> PQLPEVETIRRTLLPLIVGKTIEDVRIFWPNIIRHPRDSEAFAARMIGQTVRGLERRGKFLKFLLDRDALISHLRMEGRYAVASALEPLEPHTHVVFCFTDGSELRYRDVRKFGTMHVYAKEEADRRPPLAELGPEPLSPAFSPAVLAERAVKTK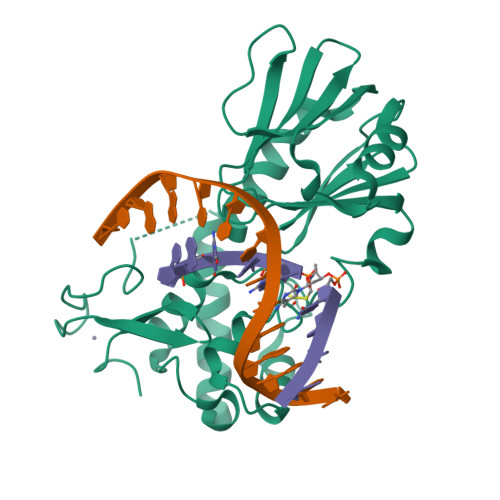RSVKALLLDCTVVAGFGNIYVDESLFRAGILPGRPAASLSSKEIERLHEEMVATIGEAVMKGGSTPRTYVNTQGEAGTFQHHLYVYGRQGNPCKRCGTPIEKTVVAGRGTHYCPRCQR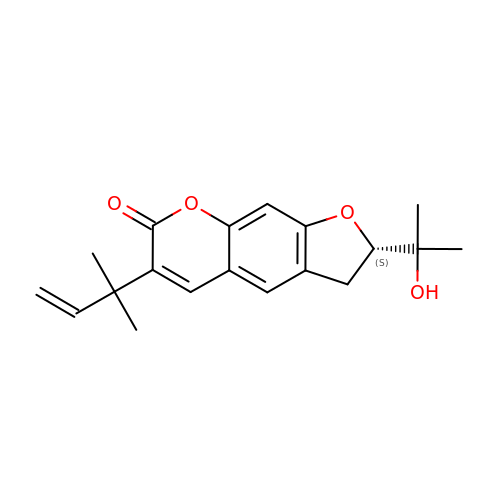6-(1,1-DIMETHYLALLYL)-2-(1-HYDROXY-1-METHYLETHYL)-2,3-DIHYDRO-7H-FURO[3,2-G]CHROMEN-7-ONE | C19 H22 O4 | JCDLLLXYAICSQV-INIZCTEOSA-N> GGSEFSDTHIFIIMGASGDLAKKKIYPTIWWLFRDGLLPENTFIVGYARSRLTVADIRKQSEPFFKATPEEKLKLEDFFARNSYVAGQYDDAASYQRLNSHMNALHLGSQANRLFYLALPPTVYEAVTKNIHESCMSQIGWNRIIVEKPFGRDLQSSDRLSNHISSLFREDQIYRIDHYLGKEMVQNLMVLRFANRIFGPIWNRDNIACVILTFKEPFGTEGRGGYFDEFGIIRDVMQNHLLQMLCLVAMEKPCSTNSDDVRDEKVKVLKCISEVQANNVVLGQYVGNPDGEGEATKGYLDDPTVPRGSTTATFAAVVLYVENERWDGVPFILRCGKALNERKAEVRLQFHDVAGDIFHQQCKRNELVIRVQPNEAVYTKMMTKKPGMFFNP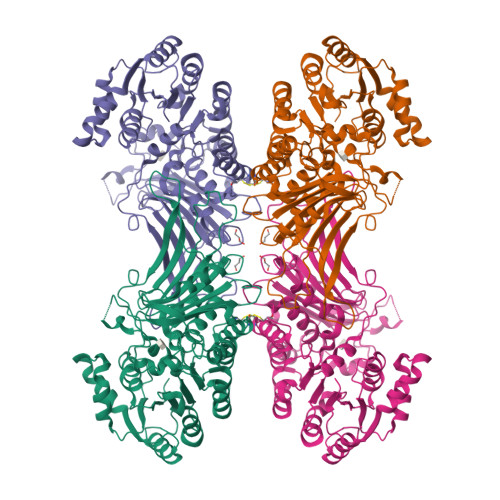EESELDLTYGNRYKNVKLPDAYERLILDVFCGSQMHFVRSDELREAWRIFTPLLHQIELEKPKPIPYIYGSRGPTEADELMKRVGFQYEGTYKWVN>REFAPPPNLPDPKFESKAALLAARGPEELLCFTERLEDLVCFWEEAASAGVGPGQYSFSYQLEDEPWKLCRLHQAPTARGAVRFWCSLPTADTSSFVPLELRVTAASGAPRYHRVIHINEVVLLDAPVGLVARLADESGHVVLRWLPPPETPMTSHIRYEVDVSAGQGAGSVQRVEILEGRTECVLSNLRGRTRYTFAVRARMAEPSFGGFWSEWSEPVSLLTPSDLD[2x];> APPRLICDSRVLERYLLEAKEAEKIT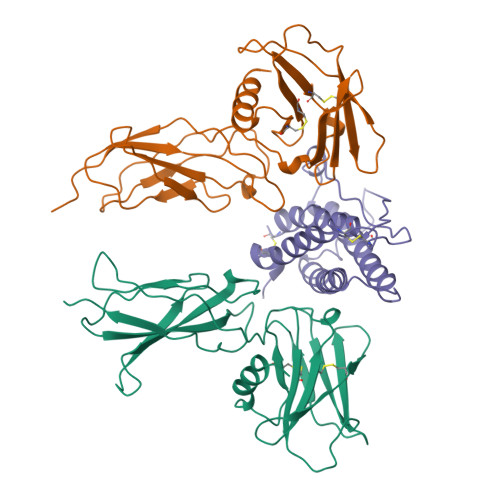TGCAEHCSLNEKITVPDTKVNFYAWKRMEVGQQAVEVWQGLALLSEAVLRGQALLVKSSQPWEPLQLHVDKAVSGLRSLTTLLRALGAQKEAISPPDAASAAPLRTITADTFRKLFRVYSNFLRGKLKLYTGEACRTGDR> GAPATVTEQGEDITSKKDRGVLKIVKRVGNGEETPMIGDKVYVHYKGKLSNGKKFDS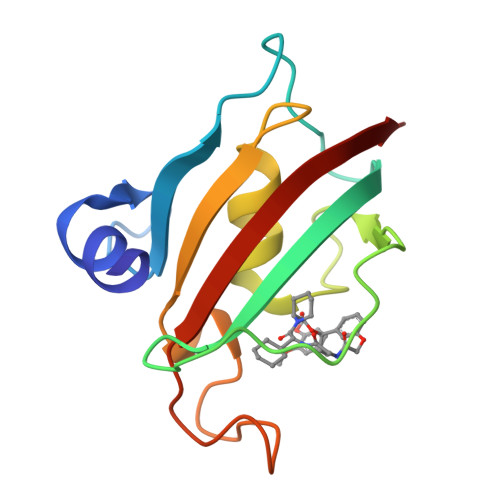SHDRNEPFVFSLGKGQVIKAWDIGVATMKKGEICHLLCKPEYAYGSAGSLPKIPSNATLFFEIELLDFKGE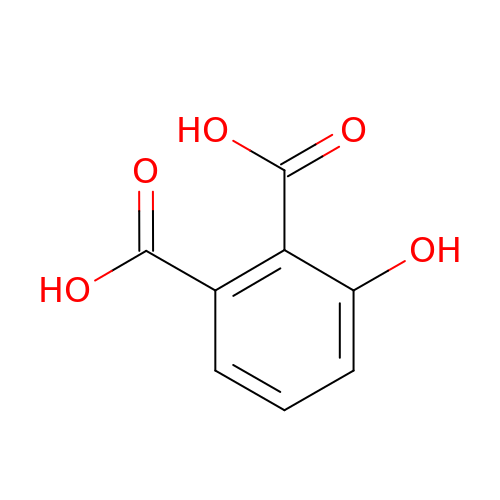3-hydroxybenzene-1,2-dicarboxylic acid | C8 H6 O5 | MNUOZFHYBCRUOD-UHFFFAOYSA-N>MKMEARQKQNSFTSKMQKIVNHRAFTFTVIALILFNALIVGIETYPRIYADHKWLFYRIDLVLLWIFTIEIAMRFLASNPKSAFFRSSWNWFDFLIVTLSLVELFL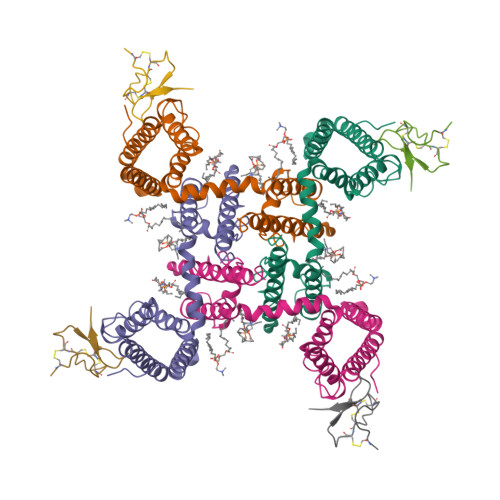ADVEGLSVLRILRVLRVLRAISVVPSLRRLVDALVMTIPALGNILILMSIFFYIFAVIGTMLFQHVSPEYFGNLQLSLLTLFQVVTLESWASGVMRPIFAEVPWSWLYFVSFVLIGTFIIFNLFIGVIVNNVEKAELTDNEEDGEADGLKQEISALRKDVAELKSLLKQSK[4x];>[4x]ECLEIFKACNPSNDQCCKSSKLVCSRKTRWCKYQI>[2x]PYPFKLPDLGYPYEALEPHIDAKTMEIHHQKHHGAYVTNLNAALEKYPYLHGVEVEVLLRHLAALPQDIQTAVRNNGGGHLNHSLFWRLLTPGGAKEPVGELKKAIDEQFGGFQA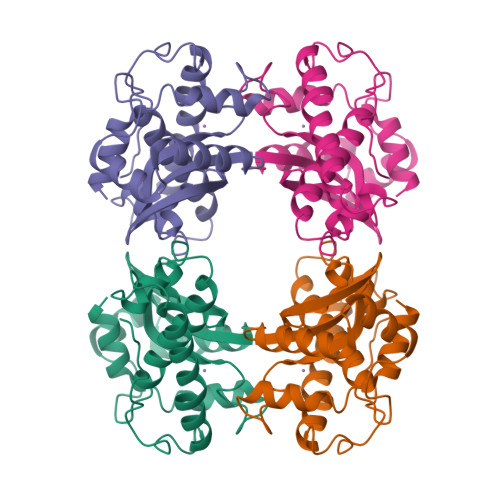LKEKLTQAAMGRFGSGWAWLVKDPFGKLHVLSTPNQDNPVMEGFTPIVGIDVWEHAYYLKYQNRRADYLQAIWNVLNWDVAEEFFKKA>[2x]SNAMTQSPIFLTPVFKEKIWGGTALRDRFGYSIPSESTGECWAISAHPKGPSTVANGPYKGKTLIELWEEHREVFGGVEGDRFPLLTKLLDVKEDTSIKVHPDDYYAGENEEGELGKTECWYIIDCKENAEIIYGH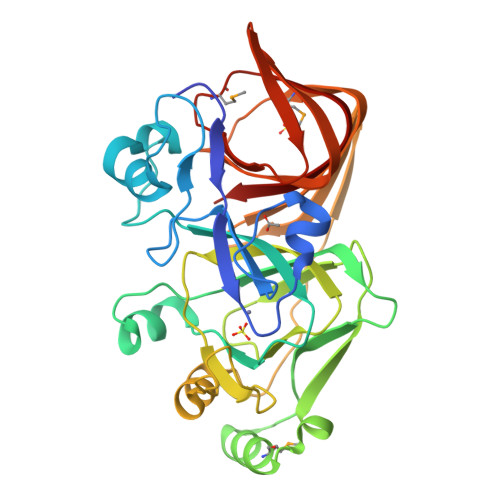TARSKTELVTMINSGDWEGLLRRIKIKPGDFYYVPSGTLHALCKGALVLETQQNSDATYRVYDYDRLDSNGSPRELHFAKAVNAATVPHVDGYIDESTESRKGITIKTFVQGEYFSVYKWDINGEAEMAQDESFLICSVIEGSGLLKYEDKTCPLKKGDHFILPAQMPDFTIKGTCTLIVSHI>SNAMLKRTPLFDLYKEYGGKTIDFGGWELPVQFSSIKKEHEAVRTAAGLFDVSHMGEVEVSGNDSLSFLQRLMTNDVSALTPGRAQYTAMCYPDGGTVDDLLIYQKGENRYLLVINASNIDKDLAWMKEHAAGDVQIDNQSDQIALLAVQGPKAEAILKNLTDADVSALKPFAFIDEADISGRKALISRTGYTGEDGYEIYCRSDDAMHIWKKIIDAGDAYGLIPCGLGARDTL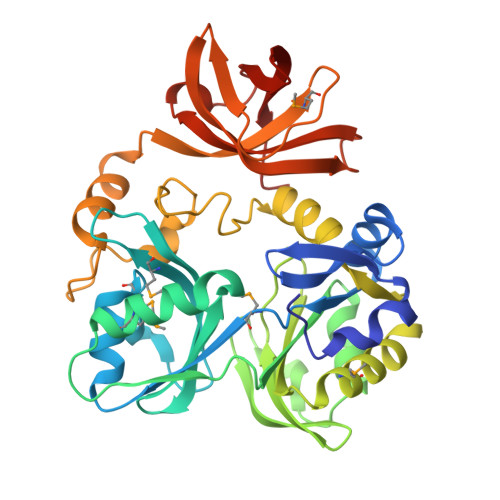RFEANIPLYGQELTRDITPIEAGIGFAVKHKKESDFFGKSVLSEQKENGAKRKLVGLEMIEKGIPRHGYEVFQNGKSVGKVTTGTQSPTLGKNVGLALIDSETSEIGTVVDVEIRKKLVKAKVVKTPFYKR[2x]3-(2-methylphenyl)propanoic acid | C10 H12 O2 | 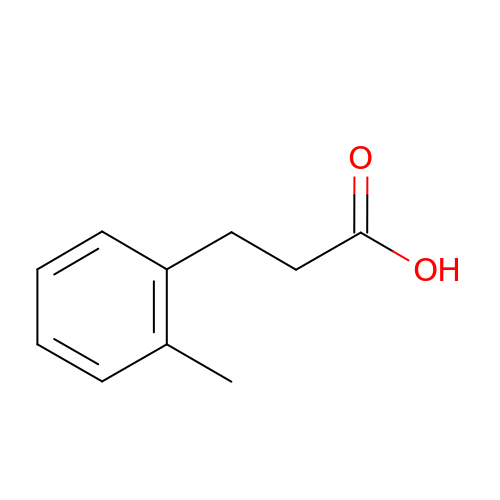JIRKNEAMPYVPTD-UHFFFAOYSA-N>[2x]MRGSHHHHHHGSMQYALLFPGQGSQCIGMGKSFYEGHTLA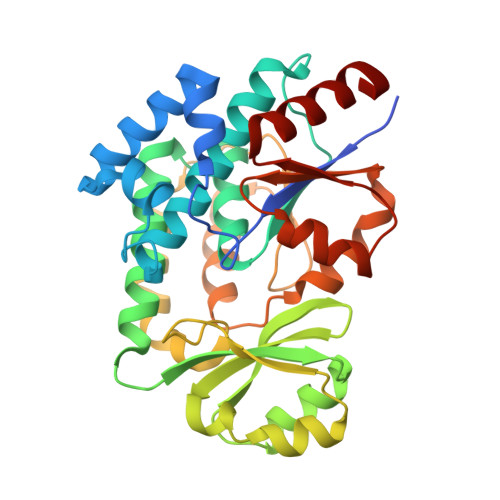KELFERASNALKVDMKKTLFEENELLKESAYTQPAIYLVSYIAYQLLNKQANGGLKPVFALGHSLGEVSAVSLSGALDFEKALKLTHQRGKMMQEACANKDASMMVVLGVSEESLLSLCQRTKNVWCANFNGGMQVVLAGVKDDLKALEPTLKEMGAKRVVFLEMSVASHCPFLEPMIFKFQELLEKSLKDKFHFEIISNATNEAYHNKAKAVELLSLQLTQPVRYQDCVKSNNDRVDIFFELGCGSVLKGLNKRLSNKPTISVGDNKGLDEAIEFLEEYV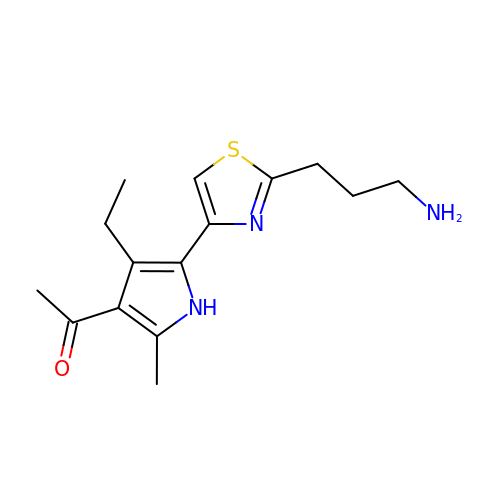1-[5-[2-(3-azanylpropyl)-1,3-thiazol-4-yl]-4-ethyl-2-methyl-1~{H}-pyrrol-3-yl]ethanone | C15 H21 N3 O S | BNBLIFSAGIHMCH-UHFFFAOYSA-N> MFENITAAPADPILGLADLFRADERPGKINLGIGVYKDETGKTPVLTSVKKAEQYLLENETTKNYLGIDGIPEFGRCTQELLFGKGSALINDKRARTAQTPGGTGALRVAADFLAKNTSVKRVWVSNPSWPNHKSVFNSAGLEVREYAYYDAENHTLDFDALINSLNEAQAGDVVLFHGWCHNPTGIDPTLEQWQTLAQLSVEKGWLPLFDFAYQGFARGLEEDAEGLRAFAAMHKELIVASSYSKNFGLYNERVGACTLVAADSETVDRAFSQMKAAIRANYSN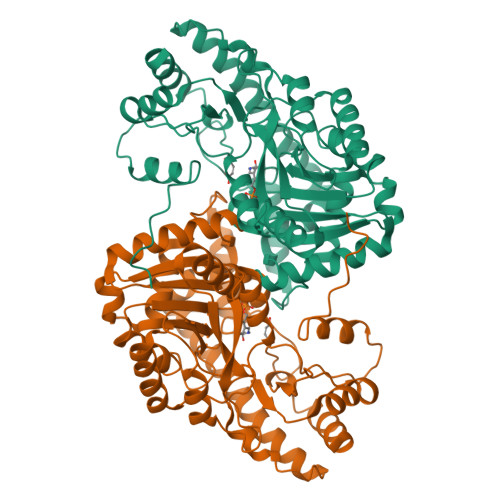PPAHGASVVATILSNDALRAIWEQELTDMRQRIQRMRQLFVNTLQEKGANRDFSFIIKQNGMFSFSGLTKEQVLRLREEFGVYAVASGRVNVAGMTPDNMAPLCEAIVAVL> MTIHSCLARRAVSVAASGARAFASGLGARAVAVGALQSARLLHTSSLRAAGAKISPSEMSRLLEERIAGWKTQTSTEEVGRVVSVGDGIARLFGLEGVQAGELVEFQNGMTGMALNLETDNVGVVIFGDDRSVLEGDSVKRTGRIVDVPIGPGLLGRVVDALGNPIDGKGPIPAKERRRVELKAPGII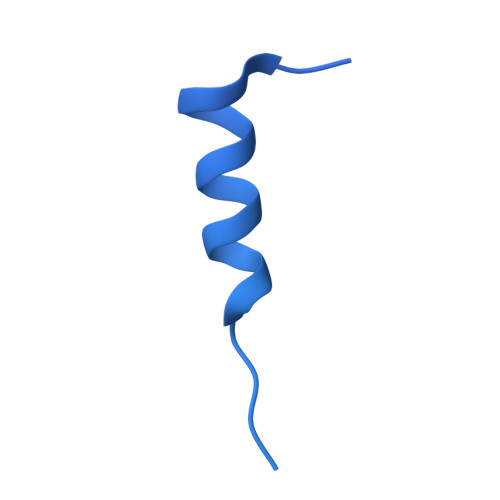PRKSVHEPMMTGLKCVDALVPVGRGQRELIIGDRQTGKTAVAVDAIINQKEINDSTDDESKKLYCIYVAVGQKRSTVAQIVKALEQRDAMKYTTVVAATASEAAPLQFLAPYSGCAMGEWFRDSGRHCVIIYDDLSKQATAYRQMSLLLRRPPGREAYPGDVFYLHSRLLERAAKMGDKSGGGSLTALPVIETQAGDVSAYIPTNVISITDGQIFLETELFYKGIRPAINVGLSVSRVGSAAQVKAMKQVAGTMKLELAQYREVAAFAQFGSDLDASTRQLLTRGTALTELLKQRQYSPMKNSVQVCVLYCGVKGYLDPLDPKEISRFESLFIDYINANHQDILKTIETEKELSEKTEAKLRAAVDEFVAMNEFKKK> GGILDPANGNSHAYFNIDEVRSKNVLKQITQLINEVTNITETFPLKPGQTTEGLVATLDAAVANFLQTGSFAISKCPIANSDPRAIDLLHEALGAVQDTGQVMIQTGRDF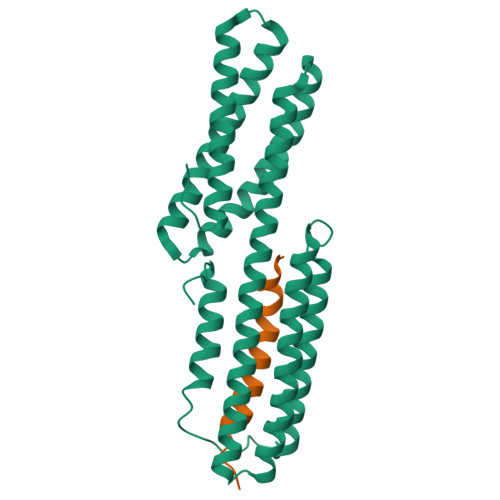VRDSTSTNKRAIATNSGRNLLTAVAKFLILADSIDVKVIVDKVDEVRETAHQMIEADTKIKVDDLYNLLISQIEELDITVRRRAIDLVKPNQRDDLLAARSALRQTAPLLYTSTRTFVRHPEHEEARRNRDYTADEMHSALNALESVLNGQQPKVTFSEYGRIGDLINE;> GGIQTSAAEATNSTTSIVEMMQMPTQQLKQSVMDLLTYEGSNDMSGLS>MPSFDVISEVDKHELTNAVDQANRELDTRFDFKGVEAKFELEDGKVINQSAPSDFQVKQMTDILRARLLARGIDVRCLEFGDVETNLAGARQKVTVKQGIEQKQAKQLVAKLKEAKLKVEAQINGDKLRVTG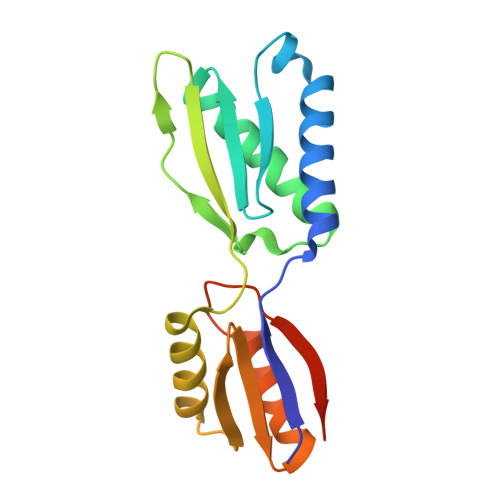KKRDDLQDAIAVLKKADFELPLQFDNFRDLEHHHHHH[2x]> RQRQK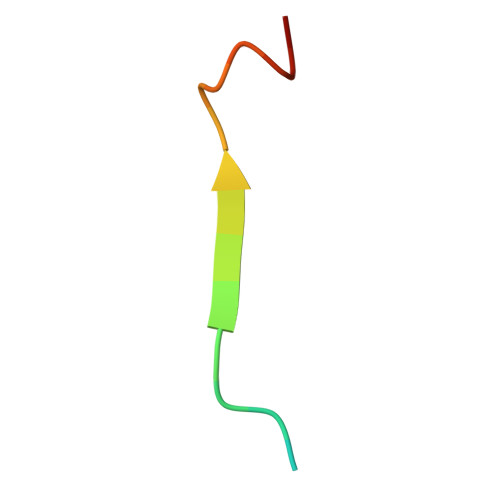RRTGALTLSGGGKRN Acinetobacter baumannii produces the catecholate siderophore acinetobactin to scavenge iron, a nutrient essential for several metabolic processes. The biosynthesis begins with BasE, a standalone adenylation domain, which activates and loads 2,3-dihydroxybenzoic acid (DHB) to the phosphopantetheinyl arm of the PCP domain of BasF. Adenylation domains have two subdomains, a large N-terminal subdomain (Acore) and a smaller C-terminal subdomain (Asub), which is highly dynamic, adopting unique conformations to carry out each individual step of the adenylation reaction. Several binding pocket residues were identified within 5 Å of the ligand, including Asn242, Phe243, Ser247, Val336, Val344, and Tyr346.

The V336A mutation that expands the binding pocket of BasE near the C4 position of DHB, resulted in a ∼13-fold improvement in apparent kcat/KM for 4-fluorosalicylic acid and a ∼76-fold improvement for 4-methylsalicylic acid. We first generated a casting of the binding pocket of WT BasE and compared its volume to V336A. We observed a significant expansion of the pocket near the region where the valine to alanine mutation was introduced, suggesting that the methyl group of 4-methylsalicylic acid was better coordinated into the mutant binding pocket as a result of this extra space. The V336A mutant bound to 4-methylsalicylic acid and the V336G mutant bound to 4-aminosalicylic acid were used to compare with the binding pocket volume of the WT enzyme. All three structures were solved in the P212121 with two molecules per asymmetric unit. No density was observed for the dynamic C-terminal subdomain, as observed in the prior BasE structures. Next, using the protein atoms from the refined structure of V336A as a search model, the structures of V336G and V336A/S247C were solved.

>[2x]MGSSHHHHHSSGENLYFQGHMKKQLIEFVRWSPERAQHYRNKGYWIDQPLTRILTVGVQSHPHSLAIICGERQLSYIELDRLSTNLATRLAEKGLGKGDTALVQLPNVAEFYIVFFALLKAGVVVLNALYSHRQYELNAFIKQIQPKLLIGSRQHEVFSNNQFIDSLHDVNLSPEIILMLNHQATDFGLLDWIETPAETFVDFSSTPADEVAFFQLSGGSTGTPKLIPRTHNDYDYSVRASAEICGLNSNTRLLCALPAPHNFMLSSPGALGVLHAGGCVVMAPNPEPLNCFSIIQRHQVNMASLVPSAVIMWLEKAAQYKDQIQSLKLLQVGGASFPESLARQVPEVLNCKLQQAFGMAEGLVNYTRLDDSDEQIFTTQGRPISSDDEIKIVDEQYREVPEGEIGMLATRGPYTFCGYYQSPEHNSQVFDEDNYYYSGDLVQRTPDGNLRVVGRIKDQINRGGEKIASEEIEKLILLHPEVMHAALVAIVDEQFGEKSCAFIVSRNPELKAVVLRRHLMELGIAQYKLPDQIKLIESLPLTAVGKVDKKQLRSILNTSTTS> MKIRFGICGLGFAGSVLMAPAMRHHPDAQIVAACDPNEDVRERFGKEYGIPVFATLAEMMQHVQMDAVYIASPHQFHCEHVVQASEQGLHIIVEKPLTLSRDEADRMIEAVERAGVHLVVGTSRSHDPVVRTLRAIVQEGSVGRVSMLNCFNYTDFLYRPRRPEELDTSKGGGIIYNQLPHQIDSIKTITGQRITAVRAMTGRLDPKRPTEGNCAAMLTLEDGACAVMVYSGYDH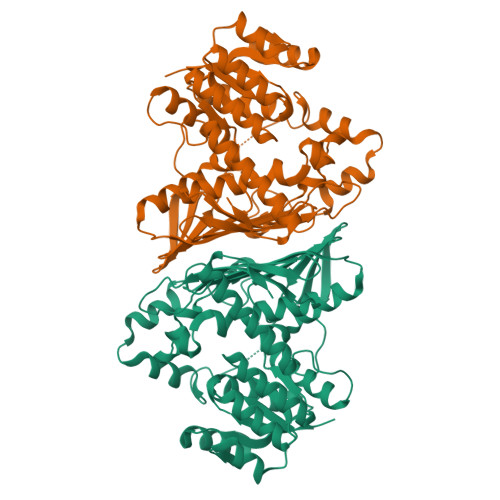FDSDEMHFWLAEGGRAKQPNHGGARKVLRQLEGDEAELRRSRYGFGGPISKSMESGNTDRKQPHFGVMLVTCEHADLRASPEGVLVYGDEGVREVPAITGRGPFSQGDTIDELRDAIAGVAPALRDARWGKDTLEVCLAVLESSATGRQVER We subsequently successfully applied our methods to the previously unknown crystal structure of the complex between synaptotagmin-1 (Syt1) and the neuronal SNARE complex, which mediates the fusion of synaptic vesicles with the synaptic membrane and is essential for Ca2+-dependent neurotransmitter release. The Syt1–SNARE complex crystallizes in two distinct crystal forms with morphologies that were indistinguishable by inspection of the crystals.

Here we have measured a synchrotron data set from a similar crystal in the same long unit cell' crystal form used for the XFEL-data derived structure. Synchrotron data were collected using the shutterless, continuous rotation method at the Northeastern Collaborative Access Team (NE-CAT) beamline at the Advanced Photon Source at Argonne National Lab on a Pilatus 6M detector (Dectris). 80 cryo-cooled crystals were screened and the best diffraction data (in the long unit cell form) were merged from three data sets collected at three different positions on a single crystal using consecutive spindle angles. Each of the three data sets contained 150 diffraction images in 0.2° frames and an exposure time of 0.2 s. The diffraction images were indexed and integrated using XDS and scaled and merged using Scala. The synchrotron diffraction data were obtained from a single crystal judged to be the best from a pool screened for optimal diffraction, and 4.1 Å was determined to be the maximum achievable limiting resolution with this particular data set. The synchrotron data extended to lower resolution (4.1 Å) and consequently provided less detailed electron density maps. The phases for the synchrotron diffraction data were determined using molecular replacement and refined in the same manner as above. Refined independently from the XFEL-data derived structure, the synchrotron data-derived structure yielded slightly better Rwork / Rfree values than the structure refined against the XFEL diffraction data truncated to the same resolution (4.1 Å). Although the synchrotron data-derived model refined to a lower Rfree value than the XFEL data-derived model (29.5% vs. 32.9%), the electron density maps calculated from the XFEL data set generally contained more information than the synchrotron data-derived maps, even when the latter were sharpened.

>GSNRRLQQTQAQVDEVVDIMRVNVDKVLERDQKLSELDDRADALQAGASQFETSAAKLKRKYW[2x];>[2x]ALSEIETRHSEIIKLENSIRELHDMFMDMAMLVESQGEMIDRIEYNVEHAVDYVERAVSDTKKAVK;>[2x]NELEEMQRRADQLADESLESTRRMLQLVEESKDAGIRTLVMLDEQGEQLDRVEEGMNHINQDMKEAEKNLKDLGK;>[2x]ARENEMDENLEQVSGIIGNLRHMALDMGNEIDTQNRQIDRIMEKADSNKTRIDEANQRATKMLG;>KLGKLQYSLDYDFQNNQLLVGIIQAAELPALDMGGTSDPYVKVFLLPDKKKKFETKVHRKTLNPVFNEQFTFKVPYSELGGKTLVMAVYDFDRFSKHDIIGEFKVPMNTVDFGHVTEEWRDLQSAEKEEQEKLGDICFSLRYVPTAGKLTVVILEAKNLKKMDVGGLSDPYVKIHLMQNGKRLKKKKTTIKKNTLNPYYNESFSFEVPFEQIQKVQVVVTVLDYDKIGKNDAIGKVFVGYNSTGAELRHWSDMLANPRRPIAQWHTLQVEEEVDAMLAV[3x]>MHGRRLGVMGGTFDPIHYGHLVAASEVADLFDLDEVVFVPSGQPWQKGRQVSAAEHRYLMTVIATASNPRFSVSRVDIDRGGPTYTKDTLADLHALHPDSELYFTTGADALASIMSWQGWEELFELARFVGVSRPGYELRNEHITSLLGQLAKDALTLVEIPALAI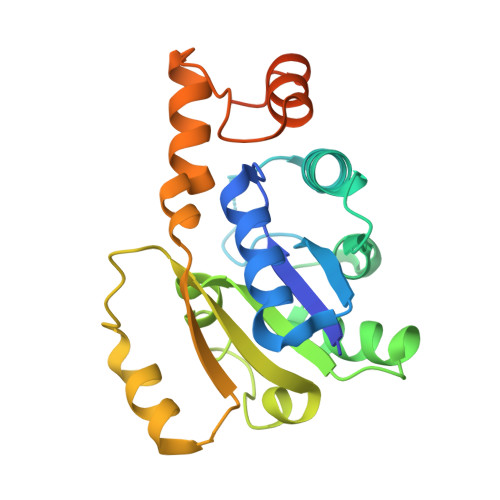SSTDCRQRAEQSRPLWYLMPDGVVQYVSKCRLYCGACDAGARSTTSLAAGNGL[2x]The RNA genome sizes of LSV1 and LSV2 are ~5.6 kb, encoding three major genes: the Orf1 with the unclear function, RdRP responsible for viral RNA replication, and the capsid protein (CP) for the host recognition and viral capsid assembly. CP forms the capsid shell that protects genomes and is responsible for both host specificity and receptor binding to transport the viral genome into infected host cells, or for intracellular trafficking. We determine cryo-EM structures of T = 4 and T = 3 capsids of virus-like particles (VLPs) of Lake Sinai virus (LSV) 2 and delta-N48 LSV1, belonging to tetraviruses, at resolutions of 2.3–2.6 Å in various pH environments. Analyses of these capsid structures reveal the intermolecular interactions that drive subunits assembly into homo-trimeric capsomeres and eventually into a complete viral capsid in which specific domains, such as the N-terminal domain, the helical domain, and the β-barrel domain/C-arm, could encapsidate nucleic acids.

The LSV2 VLPs reveal structural polymorphism of T = 4 and T = 3 particles according to EM images. From ~11,000 particle images recorded on a direct electron detector with a super-resolution mode on the FEI Titan Krios microscope, the capsid structures of LSV2 VLP within T = 4 and T = 3 architectures were determined by localized reconstructions to 2.4 and 2.6 Å resolutions on averaging around the icosahedral symmetric axes, from a respective single dataset. The T = 4 and T = 3 LSV2 VLPs show external diameters of ~492 and ~448 Å, and internal diameters of ~294 and ~250 Å, respectively, with a protein shell thickness of ~100 Å. The models of T = 4 and T = 3 LSV2 VLPs were built and refined with the homo-trimeric subunits A/B/C or D/D/D. Each icosahedral asymmetric unit (iASU) of the T = 4 particle consists of four subunits A, B, C, and D, whereas one iASU of the T = 3 particle comprises A, B, and C subunits with the C/C dimer taking up a position similar to the C/D dimer of T = 4 particles. Accordingly, the T = 4 LSV2 VLP is an icosahedral symmetrical sphere consisting of 240 copies of the 57-kDa full-length CP with 80 apparent trimeric spikes on the VLP surface, whereas the T = 3 LSV2 VLP is composed of 180 copies with 60 trimeric spikes. Long spikes (length 3.6 nm) protrude from the center of each homo-trimeric capsomere at icosahedral 3-fold (I3) and quasi 3-fold (Q3) axes in one T = 4 capsid, and at Q3 axes in one T = 3 capsid. Besides the overall differences in VLP diameters and CP numbers, the local difference in T = 4 and T = 3 architectures is that the icosahedral 2-fold (I2) axes in T = 4 particles exist between subunits B, C, and D in two sets in the quasi six-fold (Q6) arrangement but I2 axes in T = 3 particles are present along the C/C homo-dimeric capsomeres.

>MNPPTTTTTTTRTIRAPKVQLTPNSATRRRRNRRRRRPAAAIAGPLSIQPSSINRRMVSRVTRRSAVVTAAGLAWLRQYLNPMGPDTTSVTGYPDGSAVTTCIADYSNTFNVSFPPREALYCTGSSSSEKPTLVDADNYAKIDKWSNYDITLCVLALPMLRNVVMLRLYPHTPTAFALTEQTPNFPQRFPNWSVYSADGTRFNNGDEPGYLQSYVYLPNVDKHLSAARGYRLLSRGITGIFSAPALETQGFVTACQYLAEGSIQSQSIKSDAVRSVTVNSDGTVKNVESSSQTVSSMPRYVFPLDGDNCAPSSLTETYHQAYQSKATDGFYMPVLSSSRDNPFHPPQPRAIAVYGSFLARGCLDPVSEAHEADGPTHDIYRLNVADDVAPLFNTGVVWFEGISPKFSLKLKTRTVLQYIPTSGSVLANFTRHEPTYDQIALDAADRLRNLMPHAYPAAYNDWGWLGDLLDSAISMLPGVGTVYNIAKPLIKPAWNWLGNKVSDFFGNPVARDGDIFFDAK[3x]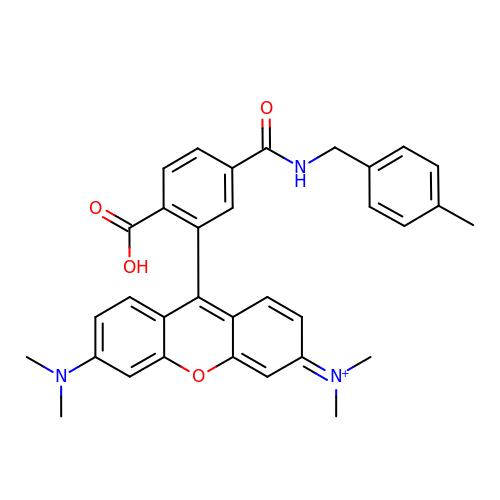[9-[2-carboxy-5-[(4-methylphenyl)methylcarbamoyl]phenyl]-6-(dimethylamino)xanthen-3-ylidene]-dimethyl-azanium | C33 H32 N3 O4 | VRTFWVCUZQBQCQ-UHFFFAOYSA-O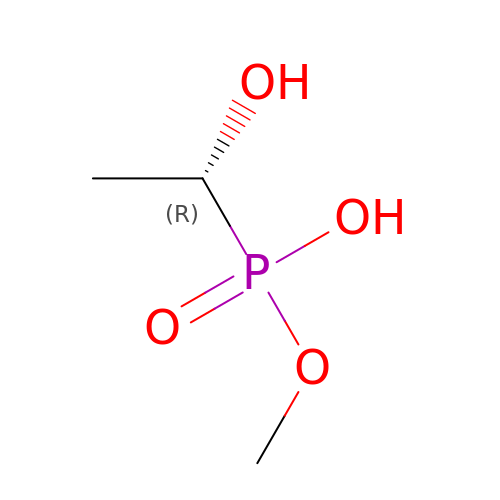methoxy-[(1~{R})-1-oxidanylethyl]phosphinic acid | C3 H9 O4 P | BAMHLGPGGHPFTF-GSVOUGTGSA-N GERANYL 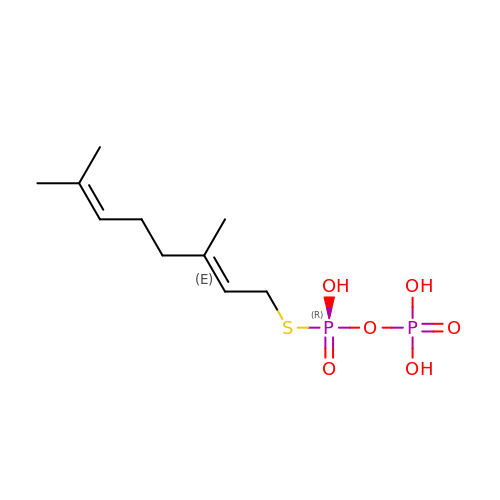S-THIOLODIPHOSPHATE | C10 H20 O6 P2 S | AKIXWSDUEPPMKM-JXMROGBWSA-N> LIIKHQMKLHLNELVDWAWRNGVTSEKFHSNNGSYVIFDHSAVVETYIINKNDLFNVTEEIEITLDKPIDYFLEKDMYGNYREHFGIAINDLLFLNTTVNI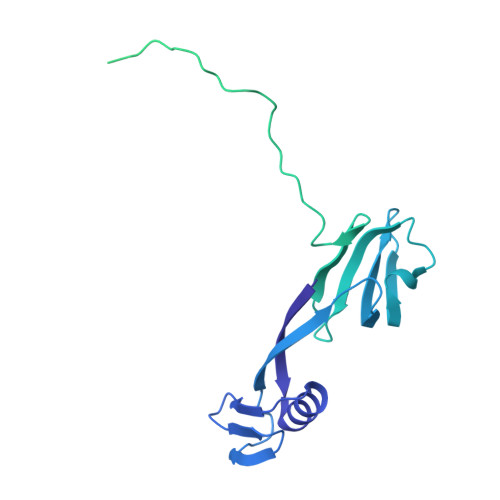WLVNDDNSHILIYKDGKLIDEYMYHQFEYEANQNKHIYPNNKASGTYPHKTEQDVTPPKKQPDTKPLPPEEHTPKVRTIKTLNGTVMKDYTPVSSIQYVKSVGIIGDSVGKGAHASYNFGDYINEKTGAKIQNLSVSSATMSEVKDNNILNQAKQLKDNELVIIQGTDDDWLFNSNAGVEVGNKITDTKTYIGAFYKVVETVKENNPKAKIVVITPTKQAKIDDTGKVIRRDTDKNKKGYTLKTYVDSQVKATKDLGLALYNAYDDSLINPYDEKFRQSSMKDGLHPTKWGHEMMYYRIAETYHKNFD>GAMEAKTLGTVTPRKPVLSVSARKIKDNAADWHNLILKWETLNDAGFTTANNIANLKISLLNKDKIELDSSSPASKENEEKVCLEYNEELEKLCEELQATLDGLTKIQVKMEKLSSTTKGICELENYHYGEESKRPPLFHTWPTTHFYEVSHKLLEMYRKELLLKRTVAKELAHTGDPDLTLSYLSMWLHQPYVESDSRLHLESMLLETGHRAL[2x]

We show that SPATA5 and SPATA5L1 associate in a DNA-binding heterohexameric complex together with heterodimeric alpha-helical proteins C1orf109 and CINP. This chromatin-associated complex, which we name 55LCC, uses ATPase activity to process replisome substrates in S-phase, facilitating their proteolytic turnover from chromatin to ensure DNA replication and mitotic fidelity. SPATA5 and SPATA5L1 belong to the CDC48 family of type II AAA+ ATPases, which contain two ATPase domains separated by an intervening sequence and an N-terminal region that typically is used to specify protein-protein interactions. We propose that 55LCC acts as an unfoldase, thereby remodeling protein complexes and facilitating their subsequent cleavage by cysteine proteases and removal from chromatin.

While little is known about C1orf109, CINP was shown to interact with DNA replication factors and was required for genome stability. CINP required expression of all other subunits for its stability but loss of CINP did not substantially affect levels of the other three members. Notably, the individual CINP and C1orf109 structures observed in the 55LCC map were nearly identical to the structures solved by X-ray crystallography and predicted by AlphaFold 2. The cryo-EM structure adopted by the C1orf109-CINP sub-complex also closely matched the T-like structure predicted by AlphaFold-Multimer35 (r.m.s.d. = 2.94 Å). In agreement with these observations, recombinantly purified CINP and C1orf109 behaved as monomers in solution while the C1orf109-CINP complex formed a stable heterodimer with a 1:1 stoichiometry and a Mw of 49.7 kDa when analyzed by native mass spectrometry. By contrast, we observed no shift for the C1orf109-CINP sub-complex in the presence of any nucleic acids. We introduced mutations in interacting residues in both C1orf109 and CINP, and tested WT and mutant proteins in co-IP experiments. Similarly, corresponding mutations at the interacting CINP residues L162, S181, and S184 impaired CINP binding to SPATA5 and SPATA5L1. Conversely, mutation of the more distal residue L178, or the conserved PRKP and RKIK motifs located at the N-terminus of CINP, did not affect complex formation.> MSSNRVLDLFKPFESFLPEVIAPERKVPYNQKLIWTGVSLLIFLILGQIPLYGIVSSETSDPLYWLRAMLASNRGTLLELGVSPIITSSMIFQFLQGTQLLQIRPESKQDRELFQIAQKVCAIILILGQALVVVMTGNYGAPSDLGLPICLLLIFQLMFASLIVMLLDELLSKGYGLGSGISLFTATNIAEQIFWRAFAPTTVNSGRGKEFEGAVIAFFHLLAVRKDKKRALVEAFYRTNLPNMFQVLMTVAIFLFVLYLQGFRYELPIRSTKVRGQIGIYPIKLFYTSNTPIMLQSALTS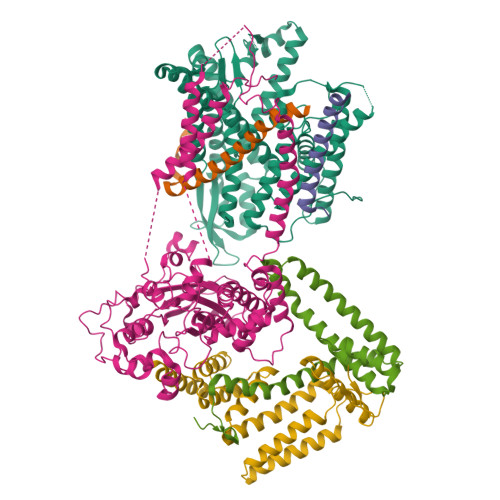NIFLISQILFQKYPTNPLIRLIGVWGIRPGTQGPQMALSGLAYYIQPLMSLSEALLDPIKTIVYITFVLGSCAVFSKTWIEISGTSPRDIAKQFKDQGMVINGKRETSIYRELKKIIPTAAAFGGATIGALSVGSDLLGTLGSGASILMATTTIYGYYEAAAKEGGFTKNLVPGFSDLM;> MSSPTPPGGQRTLQKRKQGSSQKVAASAPKKNTNSNNSILKIYSDEATGLRVDPLVVLFLAVGFIFSVVALHVISKVAGKLF;> MARASEKGEEKKQSNNQVEKLVEAPVEFVREGTQFLAKCKKPDLKEYTKIVKAVGIGFIAVGIIGYAIKLIHIPIRYVIV;> PTNYEYDEASETWPSFILTGLLMVVGPMTLLQIYQIFFGANAEDGNSGKSKEFNEEVFKNLNEEYTSDEIKQFRRKFDKNSNKKSKIWSRRNIIIIVGWILVAILLQRINSNDAIKDAATKLFDPYEILGISTSASDRDIKSAYRKLSVKFHPDKLAKGLTPDEKSVMEETYVQITKAYESLTDELVRQNYLKYGHPDGPQSTSHGIALPRFLVDGSASPLLVVCYVALLGLILPYFVSRWWARTQSYTKKGIHNVTASNFVSNLVNYKPSEIVTTDLILHWLSFAHEFKQFFPDLQPTDFEKLLQDHINRRDSGKLNNAKFRIVAKCHSLLHGLLDIACGFRNLDIALGAINTFKCIVQAVPLTPNCQILQLPNVDKEHFITKTGDIHTLGKLFTLEDAKIGEVLGIKDQAKLNETLRVASHIPNLKIIKADFLVPGENQVTPSSTPYISLKVLVRSAKQPLIPTSLIPEENLTEPQDFESQRDPFAMMSKQPLVPYSFAPFFPTKRRGSWCCLVSSQKDGKILQTPIIIEKLSYKNLNDDKDFFDKRIKMDLTKHEKFDINDWEIGTIKIPLGQPAPETVGDFFFRVIVKSTDYFTTDLDITMNMKVRDSPAVEQVEVYSEEDDEYSTDDDETESDDESDASDYTDIDTDTEAEDDESPE;> MSEFNETKFSNNGTFFETEEPIVETKSISVYTPLIYVFILVVSLVMFASSYRKKQAKKISEQPSIFDENDAHDLYFQIKEMSENEKIHEKVLKAALLNRGAESVRRSLKLKELAPQINLLYKNGSIGEDYWKRFETEVKLIELEFKDTLQEAERLQPGWVQLFVMVCKEICFNQALSRRYQSILKRKEVCIKEWELKINNDGRLVN;> MVTLEYNANSKLITASDAVVALSTETNIDQINVLTTSLIGETNPNFTPQPNEALSKMIKGLFESGMKNLQQKKLNEALKNVSLAIEMAQRKRAPWEAFAIQLPELHFMLRSKIDLCLILGKHLEALQDLDFLLGTGLIQPDVFVRKADCLLKLRQWEEARATCERGLALAPEDMKLRALLIETARNLAEYNGE>[7x]MATIAGLRGTGDWGNQERPTDFRETILWMEPNGQAPLQALMSKMSSQPTTDPEFSWWEEKLTHNRLEVKTEAAAGVTTLAVDTDQAWACVKGDILMVESVGGLWANEILKVVEDPTAGNALKVARGFAGTTAAVIPAGTFIIAIGTSFAEGSLAPKSATRNPVKLNNFCQIFKKSYEITKTADATKARTGSALANDKKRRMFDYYRDVEMAFIYGRKSETVGENGKPERTTGGLLNFITTNRTQF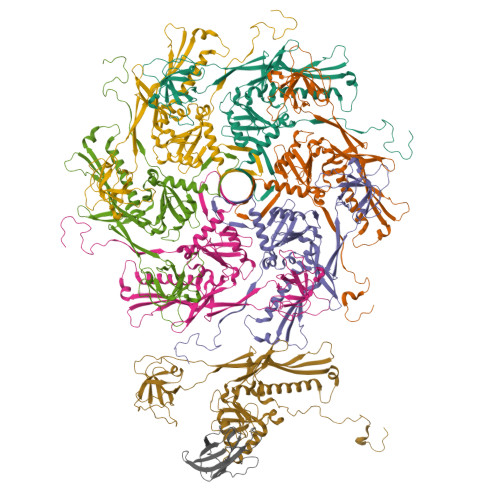GTGAGKTELTEDSLIDFFANVFNYDGQGAGNQRIAFVGNTALTKINKLARNSPSTRINFDKQVTQVYGMNFTRWVLPQGEIFFKTHPLFNVHPELSKAMMVLNPKGIKERVLRATKPENDIQQVGQDSIKGQWIGEFGLEVNHEETMAFAGGIA;> MLVHYGKLSDMPTVVDVNTTMGTDVPEDLLEIYVGCYAADGKTPAAGTGVLTFHGSWNGVHKRLIGTVDLAAAGEVIAYNPPLMFGGCKKLFVSYTGVGTQIVDVYVHRGE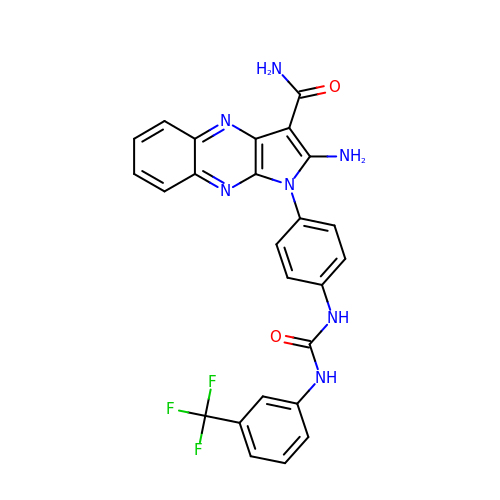2-amino-1-[4-({[3-(trifluoromethyl)phenyl]carbamoyl}amino)phenyl]-1H-pyrrolo[2,3-b]quinoxaline-3-carboxamide | C25 H18 F3 N7 O2 | RQXYLZHJULSWPX-UHFFFAOYSA-N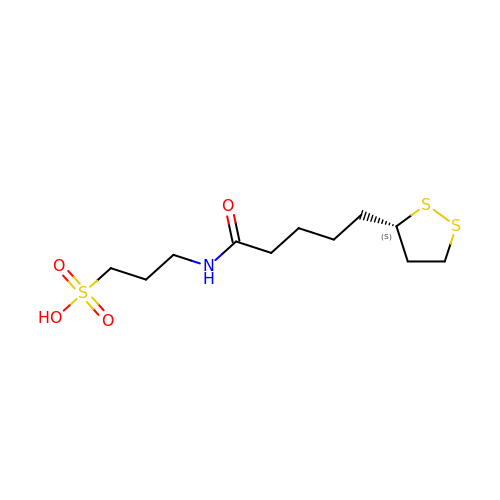3-[5-[(3~{S})-1,2-dithiolan-3-yl]pentanoylamino]propane-1-sulfonic acid | C11 H21 N O4 S3 | SZYIEKXYLQGLFW-JTQLQIEISA-N In a CRISPR-Cas system, Cas proteins form a complex with a small CRISPR RNA (crRNA) to detect and cleave invading nucleic acid (DNA or RNA) that has a complementary sequence to the crRNA. The Csm complex, with the RNA cleavage site located in Csm3 subunits, targets and cleaves ssRNA at 6-nucleotide intervals. In this study, we determined the cryo-EM structures of the Csm complex from Streptococcus thermophilus, with or without target ssRNA, at 3.3–3.5 Å. The results showed that the Csm complex displays a spiral-like architecture, with two spirally stacked density columns, including a single Cas10, a single Csm4, and multiple copies of Csm2 and Csm3.

It should be mentioned that the D33 residues in Csm3 subunits of the target ssRNA-bound state were mutated (D33A) to eliminate ssRNA cleavage. The cryo-EM micrographs and 2D class averages of both complexes display clearly a worm-like shape with mixed particle sizes. These heterogeneous particle images were classified computationally into two particle populations each yielding three-dimensional (3-D) reconstructions for the apo state (big [3.4 Å], and small [3.3 Å]) and for the target ssRNA-bound state (big [3.4 Å], and small [3.5 Å]). In total, the big maps contain 7 repeating Csm3 and 5 repeating Csm2 subunits, while the small maps contain 5 copies of Csm3 and 3 copies of Csm2. The target ssRNA is slightly less resolved but still well enough for us to trace the backbone connectivity of the core region with an apparent base-pairing to the crRNA. The heteroduplex of crRNA and target ssRNA show a repeating base pairing pattern along the spiral configurations of Csm3 and Csm2 subunits. The pattern consists of 5 base pairs, followed by a base pair disrupted by the thumb of a Csm3 or Csm4 protein. Therefore, the Csm3 or Csm4 thumb intercalates within the crRNA-ssRNA duplex at 6-nucleotide intervals. Our structure clearly shows that the DNase active site in Cas10 is located on the opposite side from the last modeled 3’-base of the ssRNA. Although the model of the 3’ flanking sequence of the ssRNA cannot be built due to its high flexibility, lowering the threshold reveals a possible locality of the 3’ flanking sequence in the map of the target ssRNA-bound state, which does not occur in the map of the apo state. Since these bases are far away from the DNase active site, the influence of the ssRNA binding to the Csm complex must be accomplished through an allosteric mechanism.

>MAILTDENYVDKAERAISLLEKDNKGNYLLTTSQIRKLLSLCSSLYDRSKERKFDELINDVSYLRVQFVYQAGREIAVKDLIEKAQILEALKEIKDRETLQRFCRYMEALVAYFKFYGGKD[3x];>[5x]MTFAKIKFSAQIRLETGLHIGGSDAFAAIGAIASPVIKDPITNIPIIPGSSLKGKMRTLLAKVYNEKVAEKPSDDSDILSRLFGNSKDKRFKMGRLIFRDAFLSNADELDSLGVRSYTEVKFENTIDRITAEANPRQIERAIRNSTFDFELIYEITDENENQVEEDFKVIRDGLKLLELDYLGGSGSRGYGKVAFEKLKATTVFGNYDVKTLNELLTAEV;> MTYKLYIMTFQNAHFGSGTLDSSKLTFSADRIFSALVLESLKMGKLDAFLAEANQDKFTLTDAFPFQFGPFLPKPIGYPKHDQIDQSVDVKEVRRQAKLSKKLQFLALENVDDYLNGELFENEEHAVIDTVTKNQPHKDGNLYQVATTRFSNDTSLYVIANESDLLNELMSSLQYSGLGGKRSSGFGRFELDIQNIPLELSDRLTKNHSDKVMSLTTALPVDADLEEAMEDGHYLLTKSSGFAFSHATNENYRKQDLYKFASGSTFSKTFEGQIVDVRPLDFPHAVLNYAKPLFFKLEV;> MKKEKIDLFYGALLHDIGKVIQRATGERKKHALVGADWFDEIADNQVISDQIRYHMANYQSDKLGNDHLAYITYIADNIASGVDRRQSNEESDEDASAKIWDTYTNQADIFNVFGAQTDKRYFKPTVLNLKSKPNFASATYEPFSKGDYAAIATRIKNELAEFEFNQAQIDSLLNLFEAILSFVPSSTNSKEIADISLAEHSRLTAAFALAIYDYLEDKGRHNYKEDLFTKASAFYEEEAFLLASFDLSGIQDFIYNIATSGAAKQLKARSLYLDFMSEYIADSLLDKLGLNRANLLYVGGGHAYFVLANTEKTVETLVQFEKDFNQFLLANFQTRLYVAFGWGSFAAKDIMSELNSPESYRQIYQKASRMISEKKISRYDYRTLMLLNRGGKSSERECEICHSVENLVSYHDQKVCDICRGLYQFSKEIAHDHFIITENEGLPIGPNACLKGVAFEKLSQESFSRVYVKNDYKAGTIKATHVFVGDYQCDEIHKYAALSKNEDGLGIKRLAVVRLDVDDLGAAFMAGFSRQGNGQYSTLSRSATFSRSMSLFFKVYINQFASDKKLSIIYAGGDDVFAIGSWQDIIAFTVELRQNFIKWTNGKLTLSAGIGLFADKTPISLMAHQTGELEEAAKGNEKDSISLFSSDYTFKFDRFITNVYDDKLEQIRYFFNHQDERGKNFIYKLIELLRNYESEEKMNVARLAYYLTRLEELTDKDERDKFKQFKKLFFKWYTNNESDRKEAELALLLYVYEIRKD>[5x]MYSTAVLLNKISPTRDGQTMTLADLQYLSFSELRKIFDDQLSWGEARHLYHETIEQKKNNRLLEARIFTRANPQLSGAIRLGIERDSVSRSYDEMFGARSSSFVKPGSVASMFSPAGYLTELYREAKDLHFSSSAYHLDNRRPDLADLTLSQSNMDTEISTLTLSNELLLEHITRKTGGDSDALMESLSTYRQAIDTPYHQPYETIRQVIMTHDSTLSALSRNPEVMGQAEGASLLAILANISPELYNILTEEITEKNADALFAQNFSENITPENFASQSWIAKYYGLELSEVQKYLGMLQNGYSDSTSAYVDNISTGLVVNNESKLEAYKITRVKTDDYDKNINYFDLMYEGNNQFFIRANFKVSREFGATLRKNAGPSGIVGSLSGPLIANTNFKSNYLSNISDSEYKNGVKIYAYRYTSSTSATNQGGGIFTFESYPLTIFALKLNKAIRLCLTSGLSPNELQTIVRSDNAQGIINDSVLTKVFYTLFYSHRYALSFDDAQVLNGSVINQYADDDSVSHFNRLFNTPPLKGKIFEADGNTVSIDPDEEQSTFARSALMRGLGVNSGELYQLGKLAGVLDAQNTITLSVFVISSLYRLTLLARVHQLTVNELCMLYGLSPFNGKTTASLSSGELPRLVIWLYQVTQWLTEAEITTEAIWLLCTPEFSGNISPEISNLLNNLRPSISEDMAQSHNRELQAEILAPFIAATLHLASPDMARYILLWTDNLRPGGLDIAGFMTLVLKESLNANETTQLVQFCHVMAQLSLSVQTLRLSEAELSVLVISGFAVLGAKNQPAGQHNIDTLFSLYRFHQWINGLGNPGSDTLDMLRQQTLTADRLASVMGLDISMVTQAMVSAGVNQLQCWQDINTVLQWIDVASALHTMPSVIRTLVNIRYVTALNKAESNLPSWDEWQTLAENMEAGLSTQQA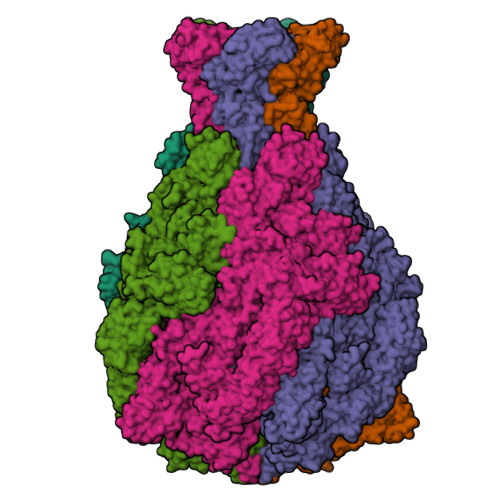QTLADYTAERLSSVLCNWFLANIQPEGVSLHSRDDLYSYFLIDNQVSSAIKTTRLAEAIAGIQLYINRALNRIEPNARADVSTRQFFTDWTVNNRYSTWGGVSRLVYYPENYIDPTQRIGQTRMMDELLENISQSKLSRDTVEDAFKTYLTRFETVADLKVVSAYHDNVNSNTGLTWFVGQTRENLPEYYWRNVDISRMQAGELAANAWKEWTKIDTAVNPYKDAIRPVIFRERLHLIWVEKEEVAKNGTDPVETYDRFTLKLAFLRHDGSWSAPWSYDITTQVEAVTDKKPDTERLALAASGFQGEDTLLVFVYKTGKSYSDFGGSNKNVAGMTIYGDGSFKKMENTALSRYSQLKNTFDIIHTQGNDLVRKASYRFAQDFEVPASLNMGSAIGDDSLTVMENGNIPQITSKYSSDNLAITLHNAAFTVRYDGSGNVIRNKQISAMKLTGVDGKSQYGNAFIIANTVKHYGGYSDLGGPITVYNKTKNYIASVQGHLMNADYTRRLILTPVENNYYARLFEFPFSPNTILNTVFTVGSNKTSDFKKCSYAVDGNNSQGFQIFSSYQSSGWLDIDTGINNTDIKITVMAGSKTHTFTASDHIASLPANSFDAMPYTFKPLEIDASSLAFTNNIAPLDIVFETKAKDGRVLGKIKQTLSVKRVNYNPEDILFLRETHSGAQYMQLGVYRIRLNTLLASQLVSRANTGIDTILTMETQRLPEPPLGEGFFANFVLPKYDPAEHGDERWFKIHIGNVGGNTGRQPYYSGMLSDTSETSMTLFVPYAEGYYMHEGVRLGVGYQKITYDNTWESAFFYFDETKQQFVLINDADHDSGMTQQGIVKNIKKYKGFLNVSIATGYSAPMDFNSASALYYWELFYYTPMMCFQRLLQEKQFDEATQWINYVYNPAGYIVNGEIAPWIWNCRPLEETTSWNANPLDAIDPDAVAQNDPMHYKIATFMRLLDQLILRGDMAYRELTRDALNEAKMWYVRTLELLGDEPEDYGSQQWAAPSLSGAASQTVQAAYQQDLTMLGRGGVSKNLRTANSLVGLFLPEYNPALTDYWQTLRLRLFNLRHNLSIDGQPLSLAIYAEPTDPKALLTSMVQASQGGSAVLPGTLSLYRFPVMLERTRNLVAQLTQFGTSLLSMAEHDDADELTTLLLQQGMELATQSIRIQQRTVDEVDADIAVLAESRRSAQNRLEKYQQLYDEDINHGEQRAMSLLDAAAGQSLAGQVLSIAEGVADLVPNVFGLACGGSRWGAALRASASVMSLSATASQYSADKISRSEAYRRRRQEWEIQRDNADGEVKQMDAQLESLKIRREAAQMQVEYQETQQAHTQAQLELLQRKFTNKALYSWMRGKLSAIYYQFFDLTQSFCLMAQEALRRELTDNGVTFIRGGAWNGTTAGLMAGETLLLNLAEMEKVWLERDERALEVTRTVSLAQFYQALSSDNFNLTEKLTQFLREGKGNVGASGNELKLSNRQIEASVRLSDLKIFSDYPESLGNTRQLKQVSVTLPALVGPYEDIRAVLNYGGSIVMPRGCSAIALSHGVNDSGQFMLDFNDSRYLPFEGISVNDSGSLTLSFPDATDRQKALLESLSDIILHIRYTIRS>SHMEQLKCCSGILKEMFAKKHAAYAWPFYKPVDVEALGLHDYCDIIKHPMDMSTIKSKLEAREYRDAQEFGADVRLMFSNCYKYNPPD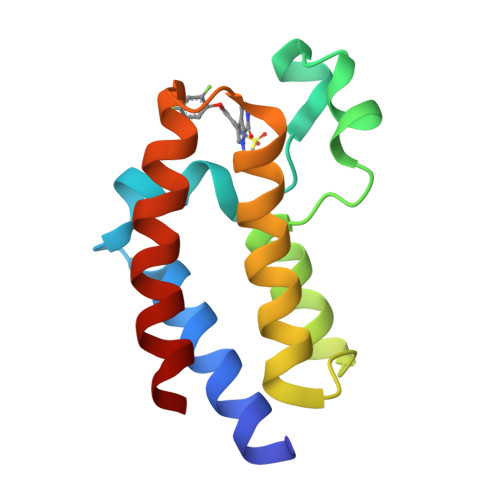HEVVAMARKLQDVFEMRFAKM[2x]> MTVGTLGVVGSAKNLKLQLSFINTRQQYVQITLFERNSFKVAEEEFSTELVEIIKTALPTLKNKKVEFEEDGDQIKQIREKGQAWVGAAEQIAPYVLPSGNITETPRNVNASNFHNPYNFVPALPRDGITGDLGDCAPAGHSYYHGDKYSGRIAVKLTTVTPLLIPDASKEEINNNHKTYPVRIGKDGKPYLPPTSIKGMLRSAYEAVTNSRLAVFEDHDSRLAYRMPATMGLQMVPARIEGDNIVLYPGTSRIGNNGRPANNDPMYAAWLPYYQNRIAYDGSRDYQMAEHGDHVRFWAERYTRGNFCYWRVRQIARHNQNLGNRPERGRNYGQHHSTGVIEQFEGFVYKTNKNIGNKHDERVFIIDRESIEIPLSRDLRRKWRELITSYQEIHKKEVDRGDTGPSAVNGAVWSRQIIADESERNLSDGTLCYAHVKKEDGQYKILNLYPVMITRGLYEIAPVDLLDETLKPATDKKQLSPADRVFGWVNQRGNGCYKGQLRIHSVTCQHDDAIDDFGNQNFSVPLAILGQPKPEQARFYCADDRKGIPLEDGYDRDDGYSDSEQGLRGRKVYPHHKGLPNGYWSNPTEDRSQQAIQGHYQEYRRPKKDGLEQRDDQNRSVKGWVKPLTEFTFEIDVTNLSEVELGALLWLLTLPDLHFHRLGGGKPLGFGSVRLDIDPDKTDLRNGAGWRDYYGSLLETSQPDFTTLISQWINAFQTAVKEEYGSSSFDQVTFIKASGQSLQGFHDNASIHYPRSTPEPKPDGEAFKWFVANEKGRRLALPALEKSQSFPIKP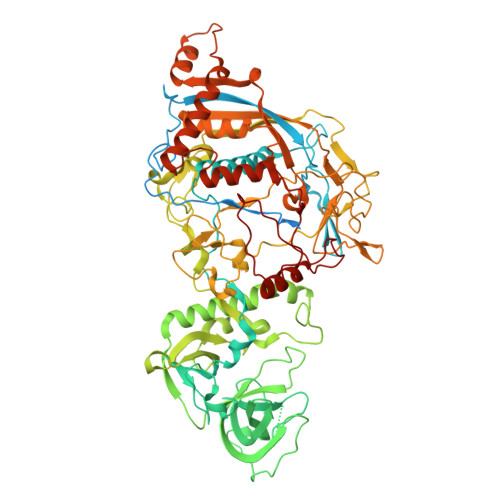S>[2x]EAPRGRAGLESGGLLAVKHPWLSAAVRLADRDGYVLSGRLSTVEHAWVLDHVVLGTVILPGTAFVELALAAADAVGLPSVSELTIEAPLALPARGAVTLQVTVEALDATGRRGFAVHSRPDGAHDAPWTAHARGVLGAAPAAATTAWAAGAWPPAGAEPVDVTRWVEALDAWVGPAFRGVTAAWRVGRSIYAD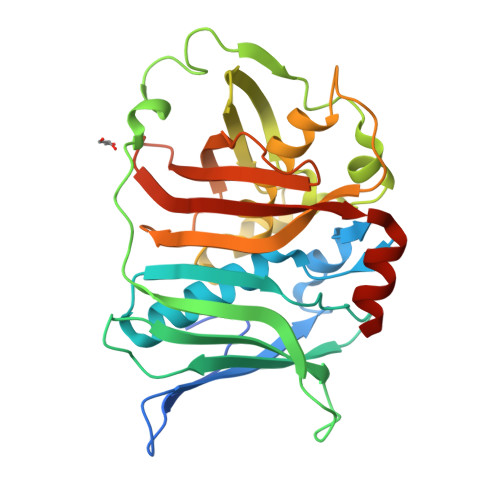LALPEGVSERAQDFGLHPALLDAALQALLRAELGAGSSPREGIPMPFAWSDVALEARGAAALRARVEVEDASDGDQLAASIELADAQGQPVARAGTFRARWATAEHVRKAAAGASERD>[2x]MGSHH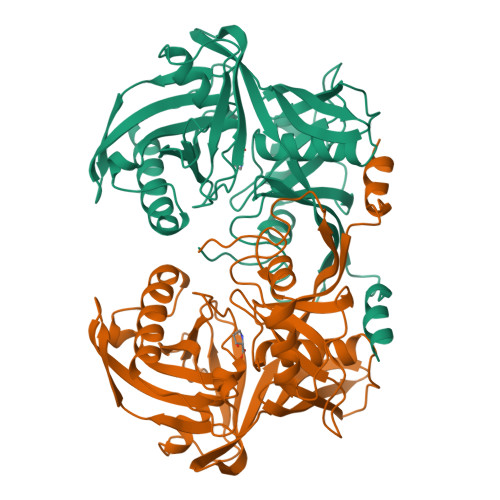HHHHSSGENLYFQGHMFKKLENLEKWEPPKDWMVIKTLDTHTAGEPLRIILSGFPEIPGKTILEKRRYLMENLDHLRKALMWEPRGHADMYGAIITEPVSEEADFGVIFMHNEGYSTMCGHATIALGKVAVECGLVEAKEPITEIKMDSPAGLIKIYVKVRDGKVEKVYFHNVPSFVLFKDETINVPGIGEVKYDLAYGGAFYAFVNAEEIGLKCTPEYYRQLIDVGMKIKRAIMSEKEIRHPFEEDLSFLYGTIFIGEPEDENSHSRHVCIFADGEVDRSPTGTGVSARLAILYEKGEIDIGEEITIESIIGTKFTGKVVEETRYGLYRAIIPEVGGNAYIVAKNTFLIDPQDPLKYGFFLR>ANSMLKGKVALVTGASRGIGRAIAKRLANDGALVAIHYGNRKEEAEETVYEIQSNGGSAFSIGANLESLHGVEALYSSLDNELQNRTGSTKFDILINNAGIGPGAFIEETTEQFFDRMVSVN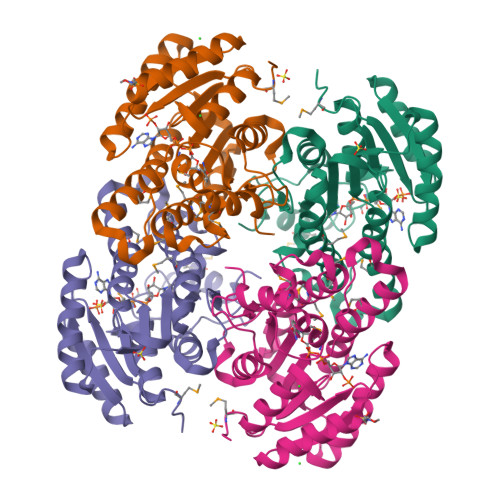AKAPFFIIQQALSRLRDNSRIINISSAATRISLPDFIAYSMTKGAINTMTFTLAKQLGARGITVNAILPGFVKTDMNAELLSDPMMKQYATTISAFNRLGEVEDIADTAAFLASPDSRWVTGQLIDVSGGSCL[2x]2,4-dibromo-6-{[(2-nitrobenzene-1-carbonyl)amino]methyl}phenyl 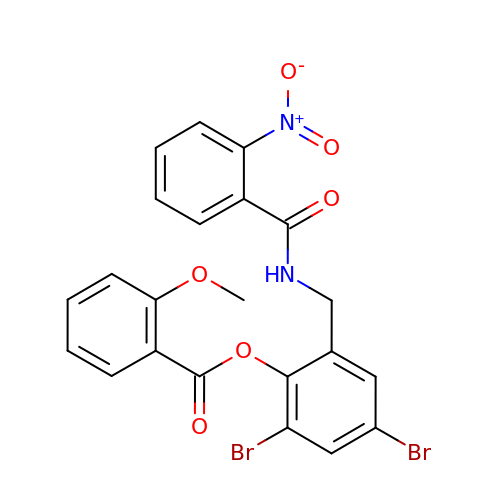2-methoxybenzoate | C22 H16 Br2 N2 O6 | UJZBVAOLSMKIHH-UHFFFAOYSA-N> MSGSSAGSSFVHLHNHTEYSMLDGAAKITPMLAEVERLGMPAVGMTDHGNMFGASEFYNSATKAGIKPIIGVEAYIAPGSRFDTRRILWGDPSQKADDVSGSGSYTHLTMMAENATGLRNLFKLSSHASFEGQLSKWSRMDAELIAEHAEGIIITTGCPSGEVQTRLRLGQDREALEAAAKWREIVGPDNYFLELMDHGLTIERRVRDGLLEIGRALNIPPLATNDCHYVTRDAAHNHEALLCVQTGKTLSDPNRFKFDGDGYYLKSAAEMRQIWDDEVPGACDSTLLIAERVQSYADVWTPRDRMPVFPVPDGHDQASWLRHEVDAGLRRRFPAGPPDGYRERAAYEIDVICSKGFPSYFLIVADLISYARSAGIRVGPGRGSAAGSLVAYALGITDIDPIPHGLLFERFLNPERTSMPDIDIDFDDRRRGEMVRYAADKWGHDRVAQVITFGTIKTKAALKDSARIHYGQPGFAIADRITKALPPAIMAKDIPLSGITDPSHERYKEAAEVRGLIETDPDVRTIYQTARGLEGLIRNAGVHACAVIMSSEPLTEAIPLWKRPQDGAIITGWDYPACEAIGLLKMDFLGLRNLTIIGDAIDNVRANRGIDLDLESVPLDDKATYELLGRGDTLGVFQLDGGPMRDLLRRMQPTGFEDVVAVIALYRPGPMGMNAHNDYADRKNNRQAIKPIHPELEEPLREILAETYGLIVYQEQIMRIAQKVASYSLARADILRKAMGKKKREVLEKEFEGFSDGMQANGFSPAAIKALWDTILPFADYAFNKSHAAGYGMVSYWTAYLKANYPAEYMAGLLTSVGDDKDKAAVYLADCRKLGITVLPPDVNESGLNFASVGQDIRYGLGAVRNVGANVVGSLLQTRNDKGKFTDFSDYLNKIDISACNKKVTESLIKAGAFDSLGHARKGLFLVHSDAVDSVLGTKKAEALGQFDLFGSNDDGTGTADPVFTIKVPDDEWEDKHKLALEREMLGLYVSGHPLNGVAHLLAAQVDTAIPAILDGDVPNDAQVRVGGILASVNRRVNKNGMPWASAQLEDLTGGIEVMFFPHTYSSYGADIVDDAVVLVNAKVAVRDDRIALIANDLTVPDFSNAEVERPLAVSLPTRQCTFDKVSALKQVLARHPGTSQVHLRLISGDRITTLALDQSLRVTPSPALMGDLKELLGPGCLGS

During DNA replication, the β-clamp interacts with DnaE1, the replicative DNA polymerase termed variously as DnaE, DnaE1, or PolC in different bacteria, greatly enhancing the processivity of the polymerase. However, mycobacteria rely on only one replicative polymerase, DnaE1. We have reported multiple lines of evidence that nargenicin acts as a DNA replication inhibitor in mycobacteria by targeting the essential DnaE1 polymerase, an enzyme identified recently as a highly vulnerable component of the DNA replication machinery in Mtb. Assessment of the antimycobacterial activity of nargenicin, a natural product that targets the replicative DNA polymerase of Staphylococcus aureus, revealed that it is a bactericidal genotoxin that induces a DNA damage response in Mycobacterium tuberculosis (Mtb) and inhibits growth by blocking the replicative DNA polymerase, DnaE1.

To elucidate the mechanism of polymerase inhibition, we determined the structure of full-length Mtb DnaE1 in complex with nargenicin and a DNA substrate by cryo-EM. The structure was determined to a resolution of 2.9 Å with well-defined density for the polymerase active site, DNA, and the bound nargenicin molecule. The cryo-EM structure of Mtb DnaE1 is identical to the previously determined crystal structure with the exception of the oligonucleotide/oligosaccharide binding (OB) domain that was not included in the crystal structure. The OB-domain is flexible as it shows a weaker density in the cryo-EM map when compared to the rest of the molecule. The DNA is bound in a canonical manner between the thumb and fingers domains, as was previously observed for other C-family DNA polymerases. The nargenicin molecule is bound in the polymerase active site and is sandwiched between the last base pair of the DNA duplex, the first base of the template strand, and the fingers domain of the polymerase. Nargenicin occupies both the position of the incoming nucleotide as well as the template base and thus mimics the position of the newly synthesized base pair. To do so, the first unpaired template base is displaced from its position and bumps into Pro668 of an adjacent helix (residues 668 to 673) that becomes disordered. On the protein side, nargenicin occupies a shallow pocket and only makes three direct contacts with the protein: Arg667 and His787 make a hydrogen bond to two oxygens in nargenicin, while Gln638 makes a hydrogen bond with the nitrogen in the pyrrole ring.> AFEVGRNVAVTEGAVVFENEYFQLLQYKPLTDKVHARPLLMVPPCINKYYILDLQPESSLVRHVVEQGHTVFLVSWRNPDASMAGSTWDDYIEHAAIRAIEVARDISGQDKINVLGFCVGGTIVSTALAVLAARGEHPAASVTLLTTLLDFADTGILDVFVDEGHVQLREATLGGGAGAPCALLRGLELANTFSFLRPNDLVWNYVVDNYLKGNTPVPFDLLFWNGDATNLPGPWYCWYLRHTYLQNELKVPGKLTVCGVPVDLASIDVPTYIYGSREDHIVPWTAAYASTALLANKLRFVLGASGHIAGVINPPAKNKRSHWTNDALPESPQQWLAGAIEHHGSWWPDWTAWLAGQAGAKRAAPANYGNARYRAIEPAPGRYVKAKALQH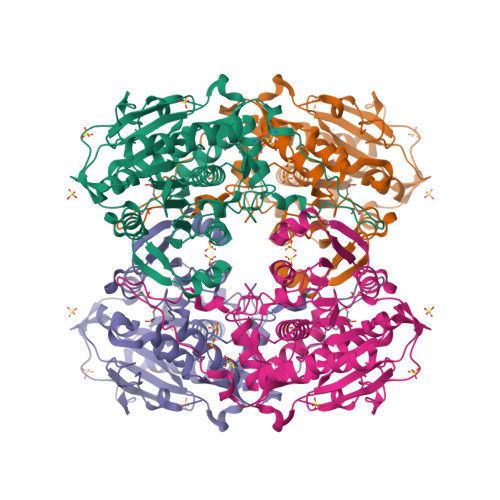HHHHH> MNEDIRTNVAESVAVQYGQASKDLHESFEIRAKSREVELTQQFLNEFNAFKAQLEKHSSEELASALKANEQALLAKQSNEVALL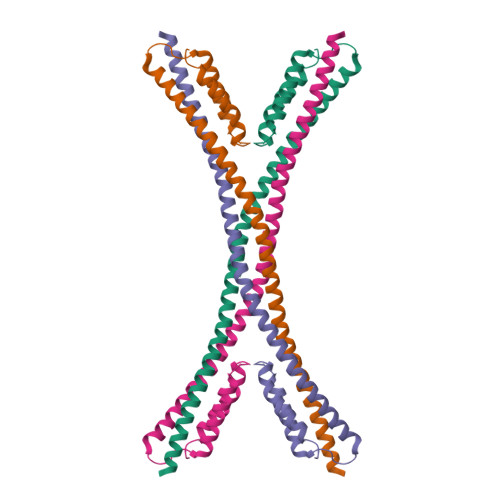SMKQVEEFTKILSEKLDQERQGRLSKLEALNGSVQELAEAVDQVDTLVMKSEVLSQLSLLTTLLKNKLHAGDESSVKIDSELARLKTLCDILPLE>[6x]MDREEMIARFAKFLREYVDDEGNEVYINRLKDLLTVTPKRSLAIDWAHLNSFDPELADELLNNPEEAIASAEDAIQIVLREPPLLVEREFKVHARFYNLPKTLLVKELGSEHINKLIQVEGIITRVSEVKPFVEKAVFVCRDCGNEMVRLQRPYENLVKPAKCDACGSRNIELDVDKSRFLNFQSFRLQDRPESLKGGQMPRFVDAILLDDLVDAALPGDRVLVTGVLRVILEQREKRPIFKKILEVNHIEQLSKEIEELEISPEDEQKIRELAKRKDIVDAIVDSIAPAIWGHRIVKKGIALALFGGVQRTLPDGTKLRGESHVLLVGDPGVAKSQLLRYVANLAPRAIYTSGKSSSAAGLTAAAVRDEFTGSWVLEAGVLVLADGGFALIDEFDKMSDRDRSAIHEALEQQTISISKAGITATLNSRTTVIAAANPKFGRFNRHKSLPEQLDLPPTLLSRFDLIFLLLDEPDEKVDASIAEHILKVRRGEAEAVTPKIPYDLLKKYIAYARKNVHPVLSREAMEEIKRYYVKMRKGLRRGDEDGVQPIPITARQLEALIRLSEAHARMRLSETVTREDARAAIEIIEAMMKTIAVDEEGNLDVSILEVGKSSKKINKIEKLVDIIKSLESEGEFGAPEEKVIEAAKQAGIGTKADIEKLLNELKSDGRVYEPRAGFYRVI

We developed an affinity-grid method employing monodispersed single particle streptavidin on a lipid monolayer to enhance particle absorption on the grid surface and alleviate sample exposure to the air-water interface. Here we generated streptavidin affinity grids with monodispersed single particle streptavidin (mspSA) on lipid monolayers, which allowed for high-resolution structure determination of challenging samples. Affinity grids could alleviate both issues by enriching the particles on to the grid and keeping them away from the AWI. Taken together, we developed mspSA affinity method which enabled the structure determination of archaea MCM and in complex with dsDNA, HIV-1 CA Di-hexamer and ScPol II EC, while providing essential insights into DNA replication initiation.

DNA replication is a fundamental process for cells, during which MCM helicases play essential roles in the initiation and elongation steps. Tko has three MCM genes (mcm1-3), among which mcm3 is the one essential for DNA replication. To enrich the MCM helicase on cryoEM grids, MCM was randomly biotinylated at its surface lysine residues. The average number of biotinylated MCM particles on the affinity grid was 316.2 per micrograph, compared to 7.5 particles per micrograph without biotinylation. We obtained a cryoEM map of MCM-apo hexamer at an overall resolution of 3.26 Å. As indicated by the local resolution, the MCM-apo is highly flexible, especially at the two peripheral MCM subunits. The MCM-apo structure shows six MCM monomers, interestingly, arranged as a left-handed open spiral. The MCM-apo forms double hexameric rings, but flexible relative to each other. The main difference between MCM-apo and MCM-ATP-dsDNA lies in the appearance of the WH motif: in MCM-apo, the WH motif shows in every other MCM monomer, i.e., B, D, and F. While in MCM-ATP-dsDNA, the WH motif shows from the second MCM to the last monomer, i.e., B, C, D, E, and F. While Tko MCM-apo constitutes a wide-open gate (20 Å), large enough to fit dsDNA, the open MCM-Cdt1-apo from human and yeast has a very narrow gate (4–6 Å).> MHHHHHHGAEIGTGFPFDPHYVEVLGERMHYVDVGPRDGTPVLFLHGNPTSSYVWRNIIPHVAPTHRCIAPDLIGMGKSDKPDLGYFFDDHVRFMDAFIEALGLEEVVLVIHDWGSALGFHWAKRNPERVKGIAFMEFIRPIPTWDEWPEFARETFQAFRTTDVGRKLIIDQNVFIEGTLPMGVVRPLTEVEMDHYREPFLNPVDREPLWRFPNELPIAGEPANIVALVEEYMDWLHQSPVPKLLFWGTPGVLIPPAEAARLAKSLPNCKAVDIGPGLNLLQEDNPDLIGSEIARWLSTLEISG

Here we describe WHaloCaMP, a modular chemigenetic calcium indicator built from bright dye-ligands and protein sensor domains. Fluorescence change in WHaloCaMP results from reversible quenching of the bound dye via a strategically placed tryptophan. WHaloCaMP is compatible with rhodamine dye-ligands that fluoresce from green to near-infrared, including several that efficiently label the brain in animals. When bound to a near-infrared dye-ligand, WHaloCaMP shows a 7× increase in fluorescence intensity and a 2.1-ns increase in fluorescence lifetime upon calcium binding.

To construct a bright, near-infrared chemigenetic Ca2+ sensor for use in animals, we focused on the JF669-HaloTag ligand. This dye-ligand has emission just on the edge of the near-infrared and has previously been reported to efficiently label neurons in mouse brains following intravascular injection. Unfortunately, the optimal range of KL–Z for bioavailability shows little overlap with the optimal range for environmental sensitivity. Thus, the excellent bioavailability of the JF669-HaloTag ligand is at the expense of environmental sensitivity; this dye-ligand does not exhibit large Ca2+-dependent fluorescence changes when used with the previously published HaloCaMP sensors. Instead of tuning the lactone–zwitterion equilibrium to find a dye with suboptimal bioavailability and environmental sensitivity, we hypothesized that we could generate Ca2+-binding-induced fluorescence changes via reversible quenching of the dye by tryptophan from the protein through PET. Mutating G171 on HaloTag7 to a tryptophan decreased fluorescence emission of bound JF669 by 85%, providing a way to strongly modulate the dye fluorescence emission. We next sought to couple the fluorescence quenching of HaloTag-bound JF669 to Ca2+-induced conformational changes in the protein. We explored different topologies of peptide calmodulin (CaM) insertions into HaloTagG171W at positions spatially proximal to the bound dye and screened for insertions that retained a high dye-ligand-capture rate close to that of HaloTag7 (above 106 M−1 s−1)17 to ensure good labeling with dye-ligand following bolus loading into complex tissue. Insertion of the myosin light-chain kinase (MLCK) CaM-binding peptide followed by CaM at position R179 of HaloTag7G171W resulted in a protein with a fast dye-ligand-capture rate and a modest Ca2+-dependent change in fluorescence.>[4x]MPYIVDV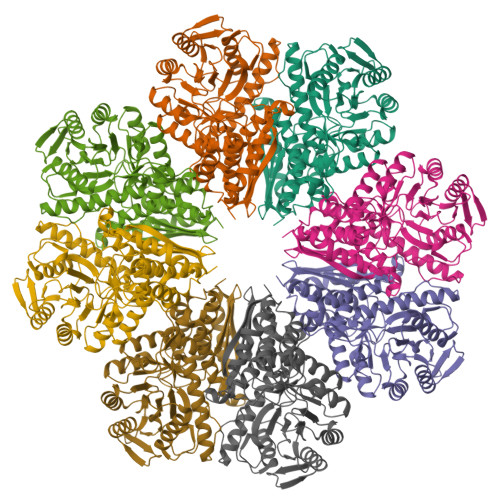YAREVLDSRGNPTVEVEVYTETGAFGRALVPSGASTGEYEAVELRDGDKDRYLGKGVLTAVNNVNEIIAPELLGFDVTEQNAIDQLLIELDGTENKGKLGANAILGVSMACARAAADFLQIPLYQYLGGFNSKTLPVPMMNIVNGGEHADNNVDIQEFMIMPVGAPNFREALRMGAQIFHSLKSVLSAKGLNTAVGDEGGFAPNLGSNEEALQTIVEAIEKAGFKPGEEVKLAMDAASSEFYNKEDGKYHLSGEGVVKTSAEMVDWYEELVSKYPIISIEDGLDENDWEGHKLLTERLGKKVQLVGDDLFVTNTKKLSEGIKNGVGNSILIKVNQIGTLTETFDAIEMAKRAGYTAVISHRSGETEDSTIADIAVATNAGQIKTGAPSRTDRVAKYNQLLRIEDQLAETAQYHGINSFYNLNK> DISEPPLHDFYCSRLLDLVFLLDGSSRLSEAEFEVLKAFVVDMMEQLRISQKWVRVAVVEYHDGSHAYIGLKDRKRPSELRRIASQVKYAGSQVASTSEVLKYTLFQIFSKIDRPEASRIALLLMASQEPQRMSRNFVRYVQGLKKKKVIVIPVGIGPHANLKQIRLIEKQAPENKAFVLSSVDELEQQRDEIVSYLCDLAPEAPPPT;> HPICEVSKVASHLEVNCDKRQLTALPPDLPKDTTILHLSENLLYTFSLATLMPYTRLTQLNLDRCELTKLQVDGTLPVLGTLDLSHNQLQSLPLLGQTLPALTVLDVSFNRLTSLPLGALRGLGE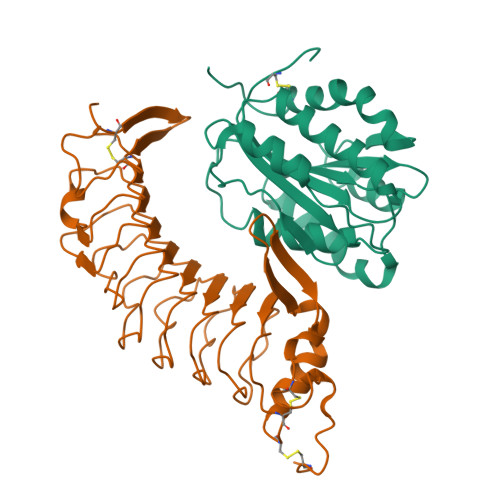LQELYLKGNELKTLPPGLLTPTPKLEKLSLANNQLTELPAGLLNGLENLDTLLLQENSLYTIPKGFFGSHLLPFAFLHGNPWLCNCEILYFRRWLQDNAENVYVWKQGVDVKAVTSNVASVQCDNSDKFPVYKYPGKGCPTLGDEGDTDLYDYYPEEDTEGDKVR> GPGYQDPGNIQIQSMPKVKERVSVPSKDDTIYSYHDSIKDSIKAVVNISTEKKIKNNFIGGGVFNDPFFQQFFGDLGG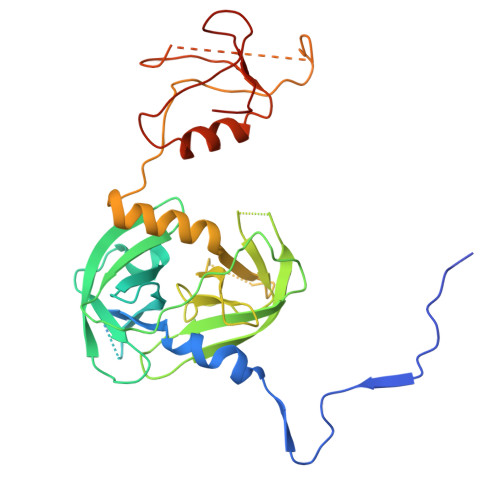MIPKERMERALGSGVIISKDGYIVTNNHVIDGADKIKVTIPGSNKEYSATLVGTDSESDLAVIRITKDNLPTIKFSDSNDISVGDLVFAIGNPFGVGESVTQGIVSALNKSGIGINSYENFIQTDASINPGNSGGALIDSRGGLVGINTAIISKTGGNHGIGFAIPSNMVKDTVTQLIKTGKIERGYLGVGLQDLSGDLQNSYDNKEGAVVISVEKDSPAKKAGILVWDLITEVNGKKVKNTNELRNLIGSMLPNQRVTLKVIRDKKERAFTLTLAERK>MKRVVITGLGIVSSIGNNQQEVLASLREGRSGITFSQELKDSGMRSHVWGNVKLDTTGLIDRKVVRFMSDASIYAFLSMEQAIADAGLSPEAYQNNPRVGLIAGSGGGSPRFQVFGADAMRGPRGLKAVGPYVVTKAMASGVSACLATPFKIHGVNYSISSASATSAHCIGNAVEQIQLGKQDIVFAGGGEELCWEMACEFDAMGALSTKYNDTPEKASRTYDAHRDGFVIAGGGGMVVVEELEHALARGAHIYAEIVGYGATSDGADMVAPSGEGAVRCMKMAMHGVDTPIDYLNSHGTSTPVGDVK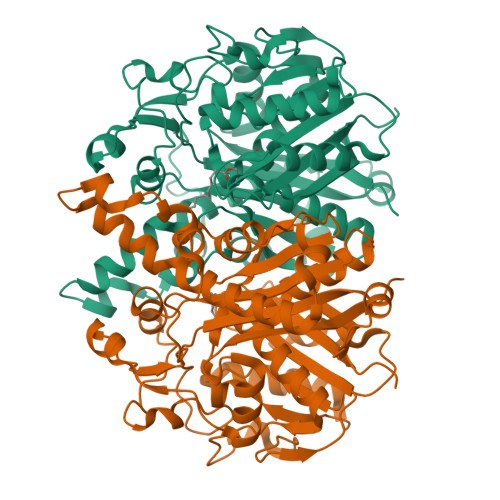ELAAIREVFGDKSPAISATKAMTGHSLGAAGVQEAIYSLLMLEHGFIAPSINIEELDEQAAGLNIVTETTDRELTTVMSNSFGFGGTNATLVMRKLKD[4x]2,2'-benzene-1,4-diylbis[6-(1,4,5,6-tetrahydropyrimidin-2-yl)-1H-indole] | C30 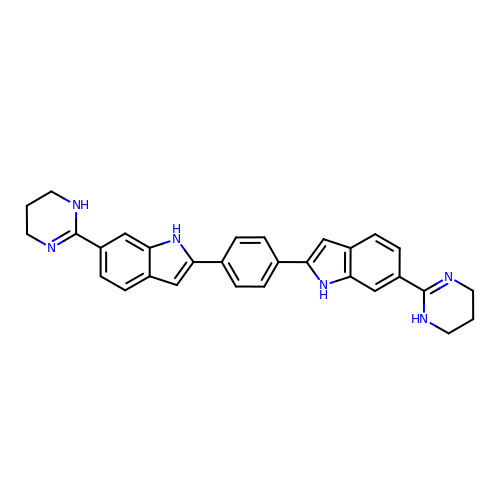H28 N6 | CYZKZDNPVSMEPI-UHFFFAOYSA-N>MASSNLLSLALFLVLLTHANSASQTSFSFQRFNETNLILQRDATVSSKGQLRLTNVNDNGEPTLSSLGRAFYSAPIQIWDNTTGAVASFATSFTFNIDVPNNSGPADGLAFVLLPVGSQPKDKGGLLGLFNNYKYDSNAHTVAVEFDTLYNVHWDPKPRHIGIDVNSIKSIKTTTWDFVKGENAEVLITYDSSTKLLVASLVYPSLKTSFIVSDTVDLKSVLPEWVIVGFTATTGITKGNVETNDILSWSFASKLSDGTTSEALNLANFALNQIL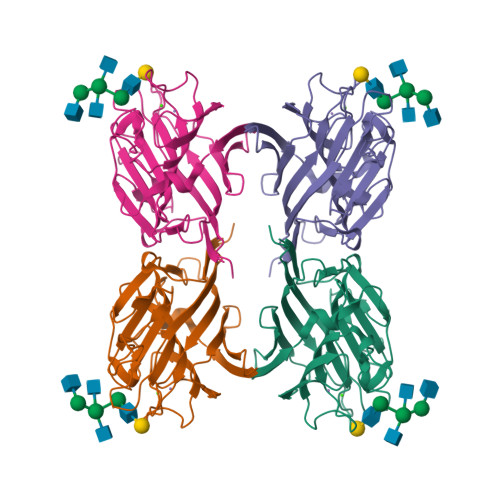[8x]> GPLGSKKHTGYVGLKNQGATCYMNSLLQTLFFTNQLRKAVYMMPTEGDDSSKSVPLALQRVFYELQHSDKPVGTKKLTKSFGWETLDSFMQHDVQELCRVLLDNVENKMKGTCVEGTIPKLFRGKMVSYIQCKEVDYRSDRREDYYDIQLSIKGKKNIFESFVDYVAVEQLDGDNKYDAGEHGLQEAEKGVKFLTLPPVLHLQLMRFMYDPQTDQN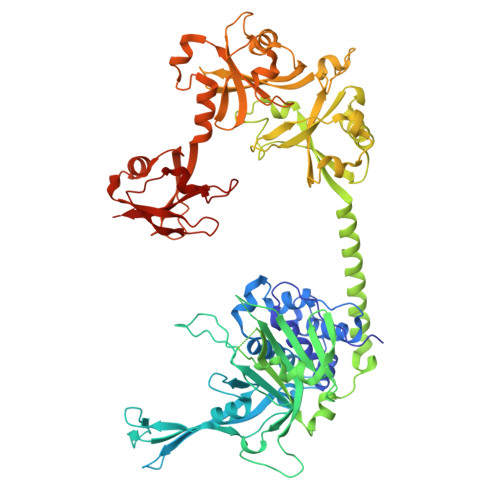IKINDRFEFPEQLPLDEFLQKTDPKDPANYILHAVLVHSGDNHGGHYVVYLNPKGDGKWCKFDDDVVSRCTKEEAIEHNYGGHDDDLSVRHCTNAYMLVYIRESKLSEVLQAVTDHDIPQQLVERLQEEKRIEAQKRKERQEAHLYMQVQIVAEDQFCGHQGNDMYDEEKVKYTVFKVLKNSSLAEFVQSLSQTMGFPQDQIRLWPMQARSNGTKRPAMLDNEADGNKTMIELSDNENPWTIFLETVDPELAASGATLPKFDKDHDVMLFLKMYDPKTRSLNYCGHIYTPISCKIRDLLPVMCDRAGFIQDTSLILYEEVKPNLTERIQDYDVSLDKALDELMDGDIIVFQKDDPENDNSELPTAKEYFRDLYHRVDVIFCDKTIPNDPGFVVTLSNRMNYFQVAKTVAQRLNTDPMLLQFFKSQGYRDGPGNPLRHNYEGTLRDLLQFFKPRQPKKLYYQQLK>MGSDKIHHHHHHMFKGIIAALWDMDSIGEIEPDVVFLLKSDILNLKFHLKILKDRGKTVFVDMDFVNGLGEGEEAILFVKKAGADGIITIKPKNYVVAKKNGIPAVLRFFALDSKAVERGIEQIETLGVDVVEVLPGAVAPKVARKIPGRTVIAAGLVETEEEARE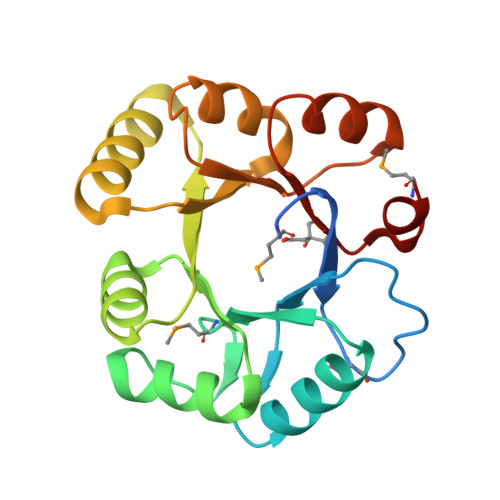ILKHVSAISTSSRILWKMKFLP[4x]>[2x]MKHHHHHHQGKITLYEDRGFQGRHYECSSDHPNLQPYLSRCNSASVDSGCWMLY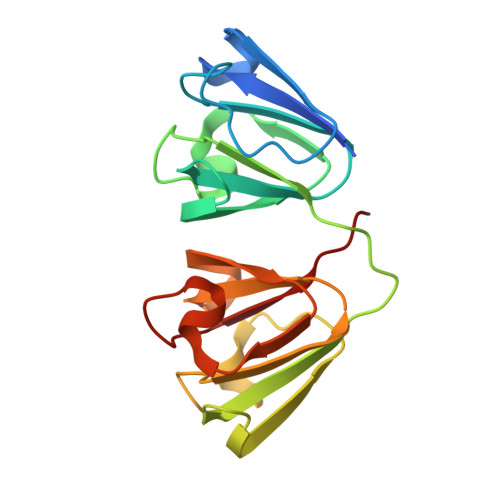EQPNYSGLQYFLRRGDYADHQQWMGLSDSVRSCRLIPHSGSHRIRLYEREDYRGQMIEFTEDCSCLQDRFRFNEIHSLNVLEGSWVLYELSNYRGRQYLLMPGDYRRYQDWGATNARVGSLRRVIDFS>[14x]MNSQNSQIQPQARYILPSFIEHSSFGVKESNPYNKLFEERIIFLGVQVDDASANDIMAQLLVLESLDPDRDITMYINSPGGGFTSLMAIYDTMQYVRADIQTVCLGQAASAAAVLLAAGTPGKRMALPNARVLIHQPSLSGVIQGQFSDLEIQAAEIERMRTLMETTLARHTGKDAGVIRKDTDRDKILTAEEAKDYGIIDTVLEYRKLSAQTA;>MSQVTDMRSNSQGLSLTDSVYERLLSERIIFLGSEVNDEIANRLCAQILLLAAEDASKDISLYINSPGGSISAGMAIYDTMVLAPCDIATYAMGMAASMGEFLLAAGTKGKRYALPHARILMHQPLGGVTGSAADIAIQAEQFAVIKKEMFRLNAEFTGQPIERIEADSDRDRWFTAAEALEYGFVDHIITRAHVNGEAQ[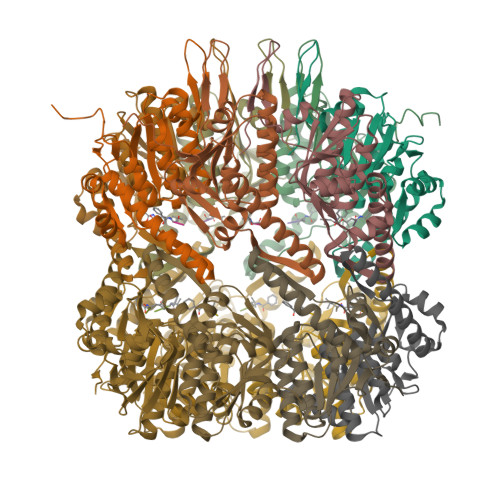14x]>[2x]MTHYTFGKEITDKQLPSQVKVAIVGAGMSGLYSAWRLQQEANCQDLAIFERSDRTGGRLDSDLIEFKNLRSDEPKTITVKEEQGGMRFLFDGMDDLMALFLKLNLQDDIVPFPMNSG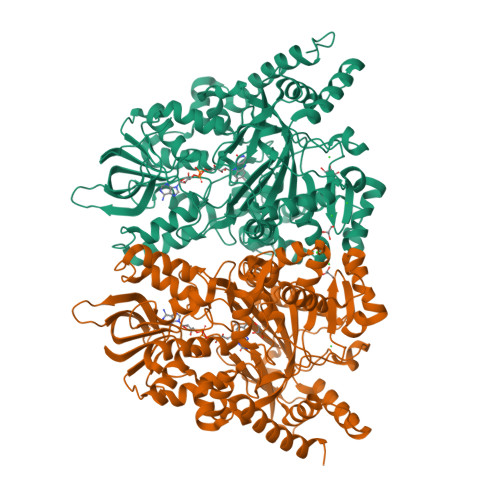GNNRLFFRGESFSVSDAQQDDYAIWSHLYNLDQSEQGVNPKDIVNVVFNRILEANPQFQQRPKVRGPQFWQDFRLECQWKGQGLNQWTLWDLYTDMGYSQECITMLYRVLGFNGTFLSQMNAGVAYQLLEDFPAGVKFKTFKDGFSTLPNKLVEEVGTNNIHLQTTIEEIDFNEESGLYELSYAHIDAHGKIHKGLVKAEKVILGLPRLALEKLFVRSNVINRLDQDRSELLWNTLQSASNQPLLKINLYYDSAWWGRGTTGRPAVEFGPNFADLPTGSVYPFYAVNEELAAALMYEERTTHPSDAVEAKLERIGNDKYERPAALTIYCDYLNINFWSNLQNIGETYHNPKQDHYVENVPDDIYPASTAVVEQATRFFKDIFNTHYVPAPVLTSARIWEGSVKFDIPANRQFGYGVHQWAVGANDKEVMATLSEPLPNLFTCGEAFSDYQGWVEGALRSTDLALEKGFGLKPLSQAYFESTHISSSDAIKAVYEENSSKLINQYIETNFAASAAPIEKADDEQSVIGVNLSYFDVK>APADNAADARPVDVSVSIFINKIYGVNTLEQTYKVDGYIVAQWTGKPRKTPGDKPLIVENTQIERWINNGLWVPALEFINVVGSPDTGNKRLMLFPDGRVIYNARFLGSFSNDMDFRLFPFDRQQFVLELEPFSYNNQQLRFSDIQVYTENIDNEEIDEWWIRGKASTHISDIRYDHLSSVQPNQNEFSRITVRIDAVRNPSYYLWSFILPLGLIIAASWSVFWLESFSERLQTSFTLMLTVVAYAFYTSNILPRLPYTTVIDQMIIAGYGSIFAAILLII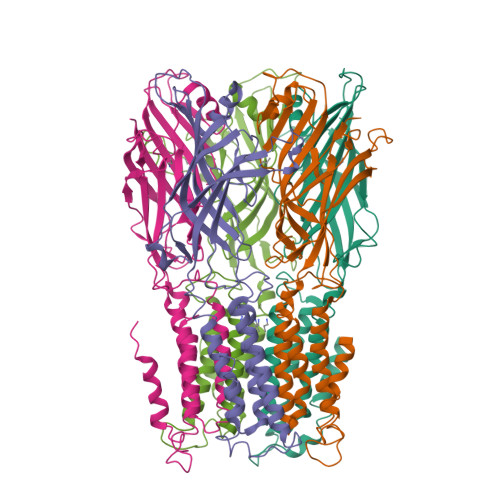FAHHRQANGVEDDLLIQRCRLAFPLGFLAIGCVLVIRGI[5x]>[6x]GSNKPPEFSFEKARVRKDSSEKKLITD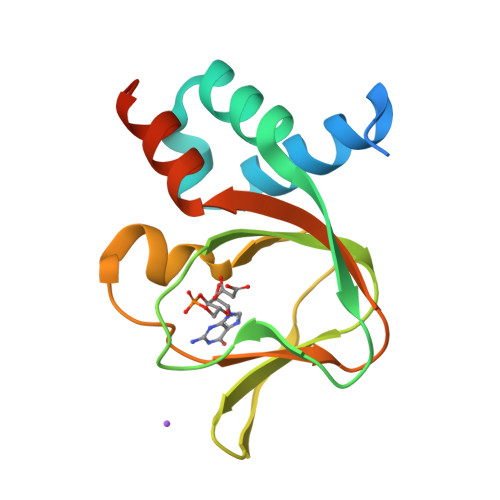ALNKNQFLKRLDPQQIKDMVECMYGRNYQQGSYIIKQGEPGNHIFVLAEGRLEVFQGEKLLSSIPMWTTFGELAILYNCTRTASVKAITNVKTWALDREVFQNIMRRTAQARDEQY N-(4-{[(2-amino-4-oxo-1,4-dihydroquinazolin-6-yl)methyl]amino}benzene-1-carbonyl)-D-glutamic 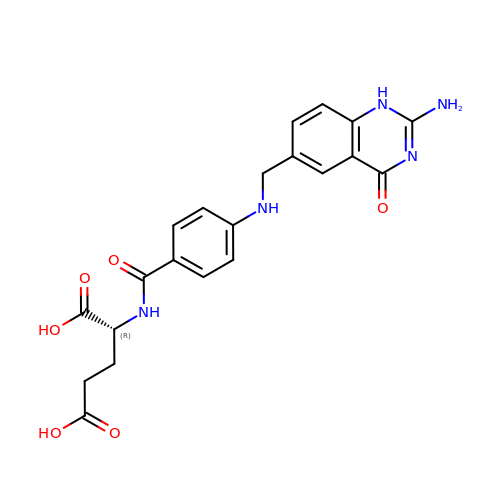acid | C21 H21 N5 O6 | UQFCLENKCDVITL-MRXNPFEDSA-N>[2x]MNQSVSSLPEKDIQYQLHPYTNARLH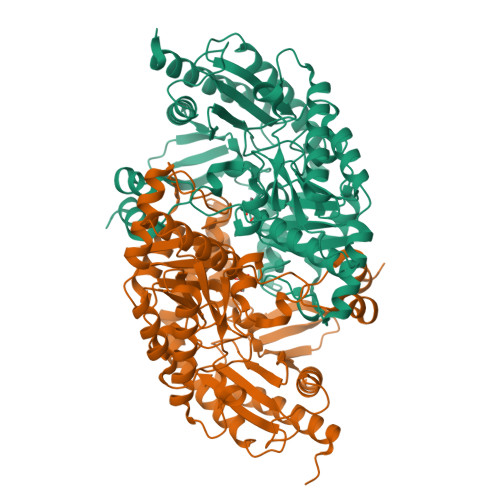QELGPLIIERGEGIYVYDDQGKGYIEAMAGLWSAALGFSNQRLIKAAEQQFNTLPFYHLFSHKSHRPSIELAEKLIEMAPVPMSKVFFTNSGSEANDTVVKMVWYLNNALGKPAKKKFISRVNGYHGITVASASLTGLPGNQRGFDLPLPGFLHVGCPHHYRFALAGESEEHFADRLAVELEQKILAEGPETIAAFIGEPLMGAGGVIVPPRTYWEKIQKVCRKYDILVIADEVICGFGRTGQMFGSQTFGIQPDIMVLSKQLSSSYQPIAAILINAPVFEGIADQSQALGALGHGFTGSGHPVATAVALENLKIIEEESLVEHAAQMGQLLRSGLQHFIDHPLVGEIRGCGLIAAVELVGDRVSKAPYQALGTLGRYMAGRAQEHGMITRAMGDAVAFCPPLIVNEQEVGMIVERFARALDDTTQWVGPGGHHHHHH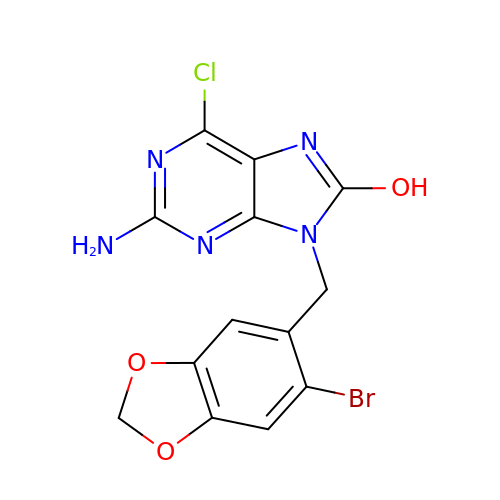2-azanyl-9-[(6-bromanyl-1,3-benzodioxol-5-yl)methyl]-6-chloranyl-purin-8-ol | C13 H9 Br Cl N5 O3 | JGUUSDOBVPWHAQ-UHFFFAOYSA-N> GIEGNFRLWDDCSSYCLVYAAPHKIYQTPLATQAVPDSPGKEGVLHYSMVMKDYVGNGQVLALRLDDFATVFVEQESLRLSLLGSDGKPRNFQYARQGAKHWSLNWLVPVGDDAPTSIKVFFKNLDGQNNILSISPLYSVEVDDKTLARWPALATFSVTQENVTQGQGLLGIRRAGVSYVAAPVNHDRHKRWSEWHSGKLLCLLDPLDAIYNYVSQNRCSLGETWEGAIYQTLAGRPVDKYAPPASKPVISQRIHFAKGNALEALTSHRVCGIPLESLARRRKPRGWEEWSSCGNPAANFVALYIATRLPFDQFRQVIHNLVHGQAVAAPDPVPLDALRTAVIEQPELARQSIAQAADIFRNYQAANPGASAAAAQQADVLAVTCPADARPCGSGASSGVLVQRENPTGAHFLNDGELPSFTVQGTQNWNLNRLQAAHLRLQVQGYVFAGYHGTSLEGAQSIVFGGIHNRQQDLEEIWRGLYVAGDPALAYGYAQDAEGDERGRIRNGTMLRVYVPRSALPRLFATSLPLDHPGASQEVARLIGHPLPLLYESITGPEAAGGNRLATILGWQLAEQAVAIPSMIPTNSRTVGNPLDPATVTLEEKQISSLPGYATKPAKDDKTEL

Pseudomonas aeruginosa can also secrete a mART toxin, known as exotoxin A (PE), but with an organization of its three functional domains (receptor, translocation, and enzymatic elements) that is opposite to DT. All these PLTs were composed of a single-chain amino acids that folded into three distinct structures: a receptor binding domain I, a translocation domain II, and a catalytic toxin domain III. Cytotoxicity associated with this family of toxins is due to their enzymatic activity and the ADP-ribosylation of eEF2. Our analysis of four of these new members by X-ray crystallography presents the defining three-domain structure typical of this family, despite substantial variability in the amino acid sequences of these proteins.

Despite having disparate levels of sequence homology, all PLTs had nearly superimposable structures compared to PE with pairwise analysis showing root-mean-square deviation (RMSD) values ranging between 2.3 Å and 3.2 Å (all atoms). Primary sequence alignment of PLT proteins indicates that K57 is conserved in Spx but not in the others. However, superposition of the crystal structures shows the presence of a comparatively positioned and positively charged lysine or arginine residue on the same β-strand (β4) in Cfx, Hmx, and Jlx. Chx266hGH, Abx259hGH, and Sfx257hGH, were the most efficient in transporting hGH across SMI-100 monolayers, while PE259hGH, Chx266hGH, Abx259hGH, Cfx259hGH, and Sfx264hGH were superior to the other PLTs for transporting hGH across AIR-100 monolayers. In comparable conditions, Hmx and Jlx appeared to be more readily cleaved by human furin, with Ahx and Spx the slowest, and PE, Chx, Cfx, and Sfx being intermediate at pH 5.5. We superposed the newly identified PLTs with PE and observed extremely high conservation and positioning of residues within the catalytic cleft, indicating that the NAD+ cofactor can be accommodated within this pocket. Remarkably, loops 1 and 2 of all PLTs superpose well with PE, whilst loop 3, which is conserved at the amino acid sequence level, presented more flexibility in our substrate-free structures and may regulate access of the catalytic site to diphthamide. Although we were not able to produce active toxins due to safety concerns, our structural analysis shows that elements involved in NAD+ binding and ADP transferase are conserved in all PLT family members, supporting their putative ADP-ribosylation activity. Only PLT genes in Aeromonas hydrophila, Chromobacterium haemolyticum, Collimonas fungivorans, and Shewanella putrefaciens matched the core gene GC content. The GC contents of three toxin genes (PE, Chx, and Cfx) showed ascending trends, while others showed descending trends, not aligning with phylogeny trees for this toxin family.> MYRTAASRARALKGVLTRSLRPARYA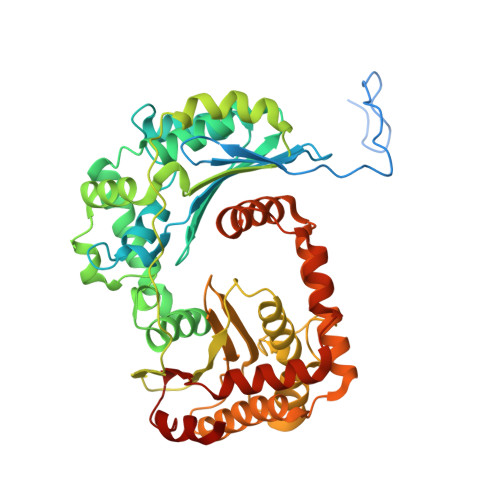SSSAVAETSSSTPAYLSWLSGGSRAALTSLDMPLQGVSLPPPLADKVEPSKLQITTLPNGLKIASETTPNPAASIGLYVDCGSIYEAPYFHGATHLLERMAFKSTLNRTHFRLVREIEAIGGNTSASASREQMSYTIDALKTYVPEMVEVLIDSVRNPAFLDWEVNEELRKMKVEIAELAKNPMGFLLEAIHSAGYSGPLASPLYAPESALDRLNGELLEEFMTENFTAARMVLAASGVEHEELLKVAEPLTSDLPNVPPQLAPKSQYVGGDFRQHTGGEATHFAVAFEVPGWNNEKEAVTATVLQMLMGGGGSFSAGGPGKGMHSWLYRRVLNEYQEVQSCTAFTSIFNDTGLFGIYGCSSPQFAAKAIELAAKELKDVAGGKVNQAHLDRAKAATKSAVLMNLESRMIAAEDIGRQILTYGERKPVDQFLKSVDQLTLKDIADFTSKVISKPLTMGSFGDVLAVPSYDTISSKFR>[2x]MFVFMLLLLLPFTISKAKDFPANPIEKAGYKLDFSDEFNGPTLDREKWTDYYLPHWCKDPESAKANYRFENGSLVEYITEDQKPWCPEHDGTVRSSAIMSFDKSWIHNFSGTTDNHERNEWRGYTTKYGYFEIRAKLSNTGGGGHQAWWMVGMQDDTNDWFN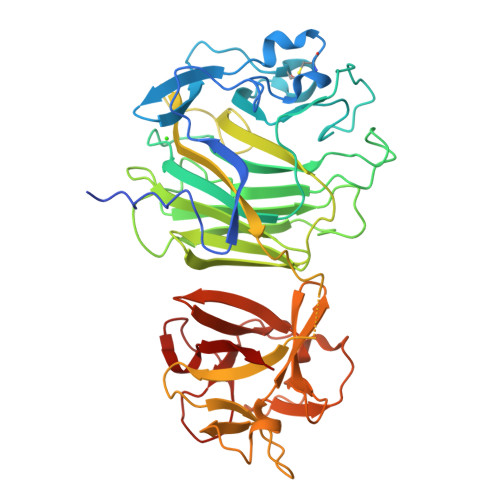SKQTGEIDILETFFSKKDTWRIAAYGWNDPNFQTSWTISEDKVPSGDPTSEYHIYAMEWTPTALKFYYDNELFKVIYGSPDYEMGTILNIYTDAGSGAHNDVWPKEWAIDYMRVWKPVDGYKESESLNNYLIRNRQTGKFLYIEENNDKVSYGDITLKNEKNAKWSKEYRDGYTLLKNNETGEYLNIENQTGYIEHGKVPKTWWSAQWSEVPVDGYTRFVNRWKPNMSIHTESYEGVLQYGNVPNTYWTSQWQLIPVE>GSKKLINDVQDVLDEQLAGLAKAHPSLTLHQDPVYVTRADAPVAGKVALLSGGGSGAEPMHCGYIGQGMLSGACPGEIFTSPTPDKIFECAMQVDGGEGVLLIIKNYTGDILNFETATELLHDSGVKVTTVVIDDDVAVKDSLYTAGRRGVANTVLIEKLVGAAAERGDSLDACAELGRKLNNQGHSIGIALGACTVPAAGKPSFTLADNEMEFGVGIHGEPGIDRRPFSSLDQTVDEMFDTLLVNGSYHRTLRFWDYQQGSWQEEQQTKQPLQSGDRVIALVNNLGATPLSELYGVYNRLTTRCQQAGLTIERNLIGAYCTSLDMTGFSITLL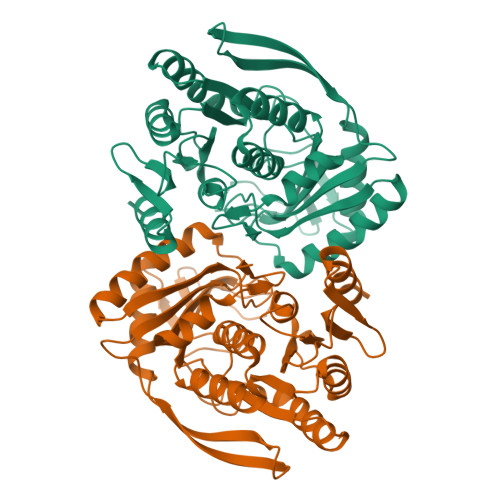KVDDETLALWDAPVHTPALNWGK[4x]>[4x]ATPVTPYYGPGHITFDWCGFGDSRSDCTNPQSPMSLDIPQQLCPKFSSKSSSSMFLSLHWNNHSSFVSYDYFNCGVEKVFYEGVNFSPRKQYSCWDEGVDGWIELKTRFYTKLYQMATTSRCIKLIQLQAPSSLPTLQAGVCRTNKQLPDNPRLALLSDTVPTSVQFVLPGSSGTTICTKHLVPFCYLNHGCFTTGGSCLPFGVSYVSDSFYYGYYDATPQIGSTESHDYVCDYLFMEPGTYNAS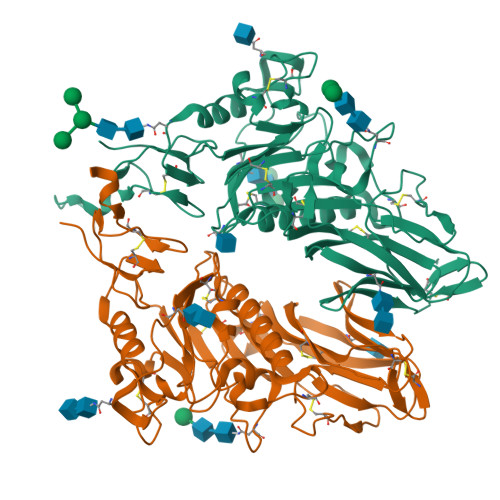TVGKFLVYPTKSYCMDTMNITVPVQAVQSIWSEQYASDDAIGQACKAPYCIFYNKTTPYTVTNGSDANHGDDEVRMMMQGLLRNSSCISPQGSTPLALYSTEMIYEPNYGSCPQFYKLFDTSGNENIDVISSSDPLVPR> MTQQMDFDAIIIGAGFGGLYSLKKLRDDFNLKVRAFDRATEVGGTWFWNQYPGALSDSETHLYCYSWDKELLQEMEIKRKYISQPDVLAYLKRVADKHDLRKDIQFETGIRSAYFDEENSFWNVTTENDEK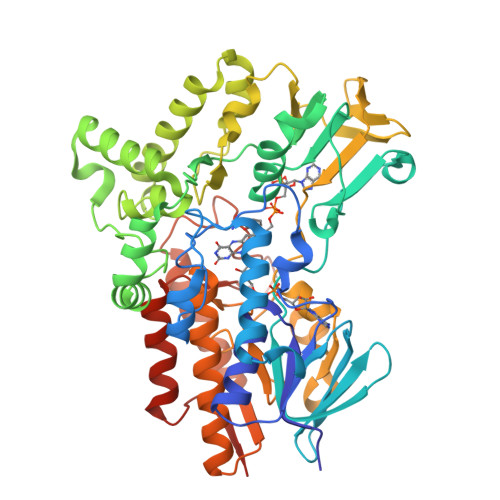FTARFLITALGLLAAPNLPKIKGIETFKGELHHTSRWPKDVTFSGKRVGVIGTGSTGVQVITAIASQVKHLTVFQRSAQYSVPIGNVVMSETDVAKIKENYDQIWENVWNSALGYGLNESTLPTMSVSAEERDKIFEKAWQEGGGFRFMFETFGDIAVDETANIEAQNFIKKKISEIVKDPFVAKKLTPTDLYACRPLCDSGYYEIFNRDNVSLEDVKANPIVEIKEDCVVTADGVEHKLDMLICATGFDAVDGSYKRIDIRGKDGISIKDHWKDGPNSYLGMMVSNFPNMFMVFGPNGPLANSPPIIETQVRWIADLIGYAEDHQINQIEATKDAVDNWTNTCSDIANKTLFAKAKCRIFGANVPGKKNTVYLYMGGLKEYRNQISEVSNNNYKGCLLKQSVKKTNLIES 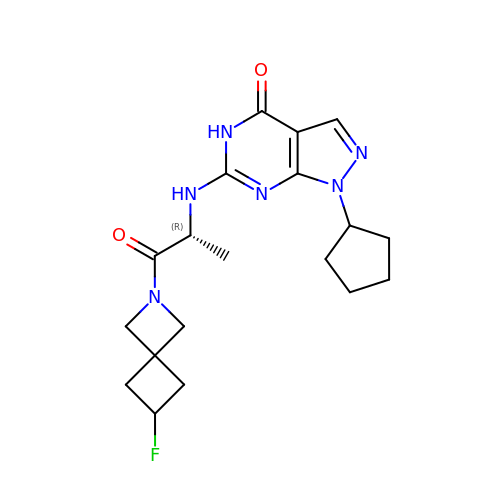1-cyclopentyl-6-[[(2R)-1-(6-fluoranyl-2-azaspiro[3.3]heptan-2-yl)-1-oxidanylidene-propan-2-yl]amino]-5H-pyrazolo[3,4-d]pyrimidin-4-one | C19 H25 F N6 O2 | GJXGHHNPNGRGBH-LLVKDONJSA-N>[8x]MTKEKISVTVDAAVLAAIDADARAAGLNRSEMIEQALRNEHL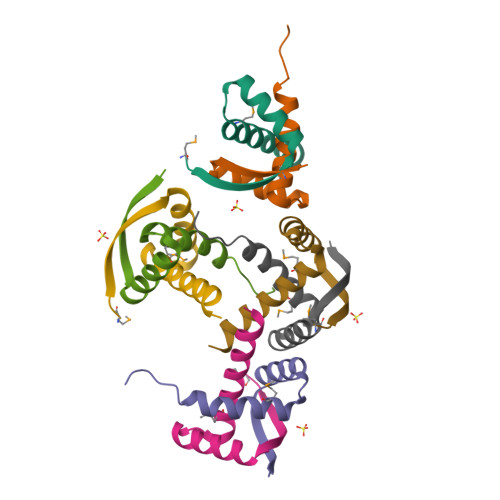RVALRDYTAKTVPALDIDAYAQRVYQANRAAGS> NLVQFGKMIECAIRNRRPALDFMNYGCYCGKGGSG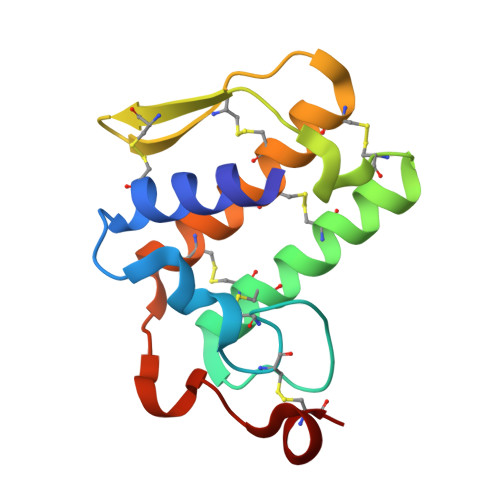TPVDDLDRCCQVHDECYAEAEKHGCYPSLTTYTWECRQVGPYCNSKTQCEVFVCACDFAAAKCFAQEDYNPAHSNINTGERCK(4-{(E)-[(5-AMINOPENTYL)IMINO]METHYL}-5-HYDROXY-6-METHYLPYRIDIN-3-YL)METHYL 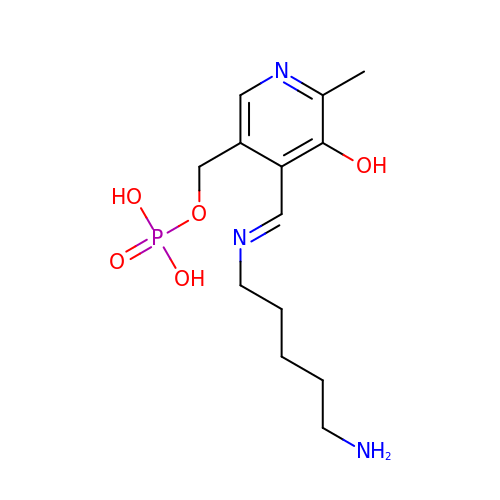DIHYDROGEN PHOSPHATE | C13 H22 N3 O5 P | NPYALNYUWCUSTP-OVCLIPMQSA-N> MSNQALYEKLEQTRTILSVKLAELINMTTIADRNDDDEGSFAQENSELAVATTSVMMVNNQTMQLIKNVQDLLILTRSIKEKWLLNQIPVTEHSK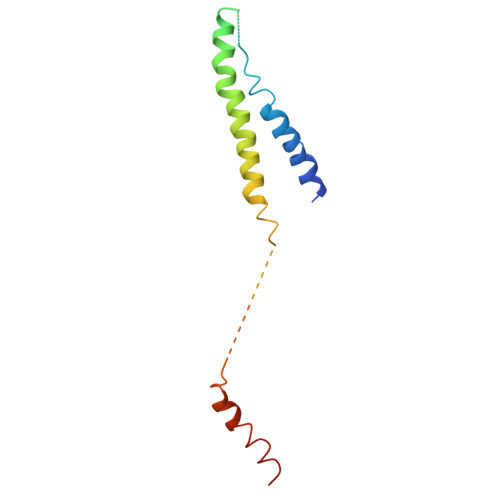VTRFDEKQIEELLDNCIETFVAEKTT>[4x]TRDQNGTWEMESNENFEGYMKALDIDFATRKIAVRLTQTKVIDQDGDNFKTKTTSTFRNLDVDF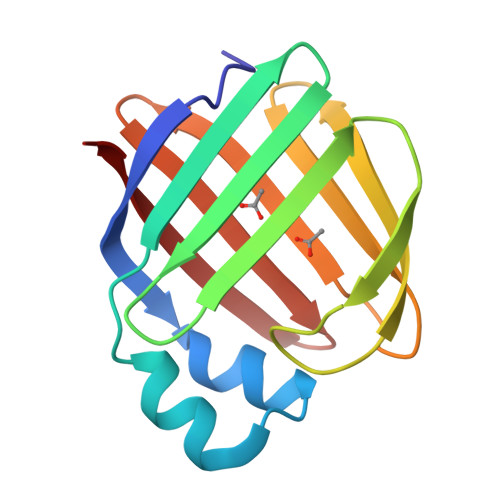TVGVEFDEYTKSLDNRHVKALVTWEGDVLVCVQKGEKENRGWKQWIEGDKLYLELTCGDQVCRQVFKKK Crc controls the sequential assimilation of amino acids and inhibits the expression of several genes involved in uptake and catabolism of sugars, alkanes and benzoate. Thus Crc protein seems to operate at the crossroad of metabolism and virulence in P. aeruginosa. Crc shares sequence similarity (25 to 37% identity) with DNA repair enzymes belonging to the family of apurinic/apyrimidinic (AP) endonucleases of both Prokaryotes and Eukaryotes. However, Crc does not appear to have nuclease activity.

Here, we report the crystal structure of the P. aeruginosa Crc refined to 1.8 Å. The crystals of Crc diffracted to 1.8 Å resolution and belonged to space group P3221 (unit-cell parameters a = b = 74.66, c = 123.16 Å), with the asymmetric unit containing one molecule. Crc is a compact, globular αβ-protein, consisting of two six-stranded β-pleated sheets flanked by six α-helices forming a four-layered αβ-sandwich motif. The overall structure of Crc shares high similarity with members of the AP endonuclease protein family. Four conserved catalytically active residues (Asp210, Asn212, Asp283 and His309 for hApe1), located in the cleft on the edge of the αβ-sandwich, are a determinant for AP endonuclease activity. Among them only two (Asp220 and His246) are present in Crc. The bulky side-chain of Tyr150 (corresponds to Asn212 in hApe1) protrudes into the active site, occupying the position of the scissile phosphate group of the DNA backbone in the apurinic/apyrimidinic site. The substitution of this residue to a serine in Crc makes DNA hydrolysis rather unlikely, which is consistent with the previously reported lack of exo- and endonuclease activity of Crc. With the exception of Arg37 (corresponding to Lys98 in hApe1) these positively charged residues are not present in Crc. Most likely, this results in a reduced capacity of Crc to attract negatively charged nucleic acids.

> GPAMRIISVNVNGIQAAAERGLLSWLQAQNADVICLQDTRASAFDLDDPSFQLDGYFLYACDAELPEQGGVALYSRLQPKAVISGLGFETADRYGRYLQADFDKVSIATLLLPSGQSGDESLNQKFKFMDDFTHYLSKQRRKRREYIYCGSLYVAHQKMDVKNWRECQQMPGFLAPERAWLDEVFGNLGYADALREVSREGDQFSWWPDSEQAEMLNLGWRFDYQVLTPGLRRFVRNAKLPRQPRFSQHAPLIVDYDWQLSI>[2x]ATGSRPRDCLDVLLS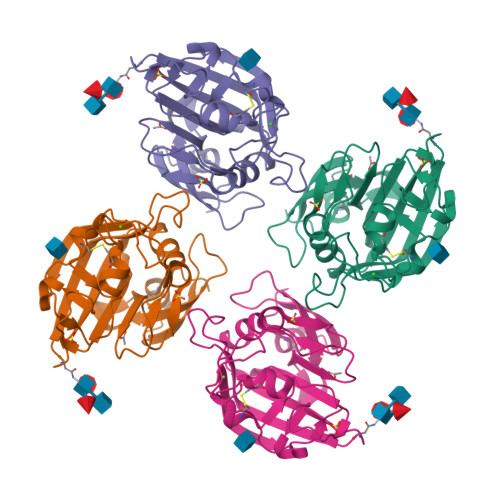GQQDDGVYSVFPTHYPAGFQVYCDMRTDGGGWTVFQRREDGSVNFFRGWDAYRDGFGRLTGEHWLGLKRIHALTTQAAYELHVDLEDFENGTAYARYGSFGVGLFSVDPEEDGYPLTVADYSGTAGDSLLKHSGMRFTTKDRDSDHSENNCAAFYRGAWWYRNCHTSNLNGQYLRGAHASYADGVEWSSWTGWQYSLKFSEMKIRPVREDR> TSLKPTAIESCMVKFELSSSKWHMTSPKPHCVNTTSDGKLKILQSGTYLIY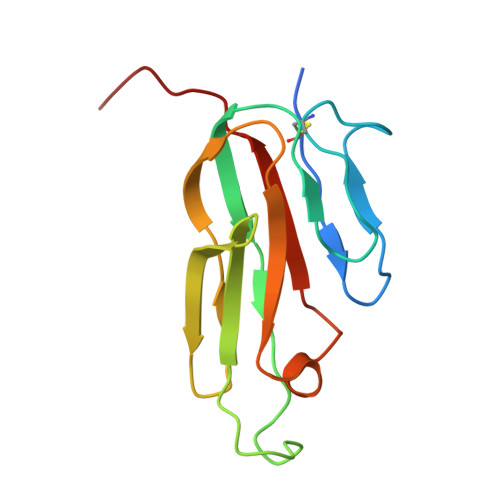GQVIPVDKKYIKDNAPFVVQIYKKNDVLQTLMNDFQILPIGGVYELHAGDNIYLKFNSKDHIQKTNTYWGIILMPDLPFIS The chloroplast envelope Quinone Oxidoreductase Homolog (ceQORH; At4g13010; molecular weight 34,034 Da) from Arabidopsis thaliana is associated to the inner membrane of the chloroplast envelope where it represents 1–2% of the crude envelope proteins. Despite its original annotation as a “QOR,” ceQORH is inactive on quinones but preferentially reduces γ-ketols in the presence of NADPH. γ-ketols are long-chain reactive electrophile oxylipins and are potentially toxic. The ceQORH monomer is formed of two domains with (i) the catalytic domain including residues from Gly3 to Pro132 and from Leu277 to Pro329 and (ii) the cofactor binding domain (Val133 to Leu276) showing the classical motif of Rossmann fold. In the ceQORH structure, the internal chloroplast targeting sequence is folded as a two anti-parallel β-strands (Thr71 to Gly81 and Asp91 to Leu97) connected by a long loop (Ser82 to Gly90).

In the crystals of the binary and ternary complexes ceQORH-13-KOTE and ceQORH-NADP+-13-KOTE, the asymmetric unit contains 12 and 8 ceQORH molecules, respectively. The quality of the electron density map for 13-KOTE differs depending on the monomers in the binary and ternary complexes, suggesting flexibility of the 13-KOTE aliphatic chain. The 13-KOTE binding site is large and solvent accessible. Upon 13-KOTE binding, the loop from Leu97 to Gly103 moves, thus stabilizing the ligand. In the complexes ceQORH-13-KOTE and ceQORH-NADP+-13-KOTE complexes, residues of three ceQORH monomers interact with 13-KOTE by hydrogen bonds and van der Waals interactions. The 13-KOTE carboxylate group from one monomer is hydrogen bonded to the Arg58 guanidinium group and Tyr14 hydroxyl group from another monomer. Thus, the 13-KOTE carboxylate group is an anchoring point allowing for oligomerization in the crystals. When the apo-ceQORH structure is compared either to the ceQORH-13-KOTE or ceQORH-NADP+-13-KOTE structure, the main chain from Asn46 to Leu61 and from Ile250 to Lys269, containing the α-helix Pro254-Met267 involved in the dimer interface, are shifted. 13-KOTE is not a substrate of ceQORH though it displays an unsaturated double bond in α,β of a carbonyl group. The tetramers observed in the crystals do not have any physiological significance.

>[12x]MAGKLMHALQYNSYGGGAAGLEHVQVPVPTPKSNEVCLKLEATSLNPVDWKIQKGMIRPFLPRKFPCIPATDVAGEVVEVGSGVKNFKAGDKVVAVLSHLGGGGLAEFAVATEKLTVKRPQEVGAAEAAALPVAGLTALQALTNPAGLKLDGTGKKANILVTAASGGVGHYAVQLAKLANAHVTATCGARNIEFVKSLGADEVLDYKTPEGAALKSPSGKKYDAVVHCANGIPFSVFEPNLSENGKVIDITPGPNAMWTYAVKKITMSKKQLVPLLLIPKAENLEFMVNLVKEGKVKTVIDSKHPLSKAEDAWAKSIDGHATGKIIVEP>SNAMVHDSALPFDALPMPPQGREGFEECPYLDSQWVADTNGQRMTGQGVDTRFDTPACVFWSYPEAPQATVMVRH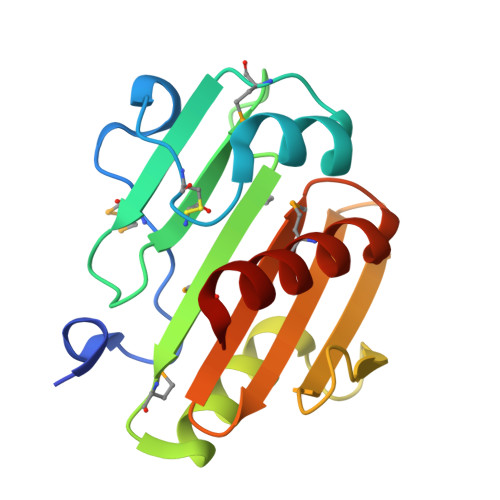MPSEEEAIRVVDWAAPIDTTEPAEEPDGWSGGRAGHEEGAVYAVQKGPVAVVVWSNQQQSLKAELMAKEAIARLGL[2x]>[2x]MRVLIVKTSSMGDVLHTLPALTDAQQAIPGIKFDWVVEEGFAQIPSWHAAVERVIPVAIRRWRKAWFSAPIKAERKAFREALQAKNYDAVIDAQGLVKSAALVTRLAHGVKHGMDWQTAREPLASLFYNRKHHIAKQQHAVERTRELF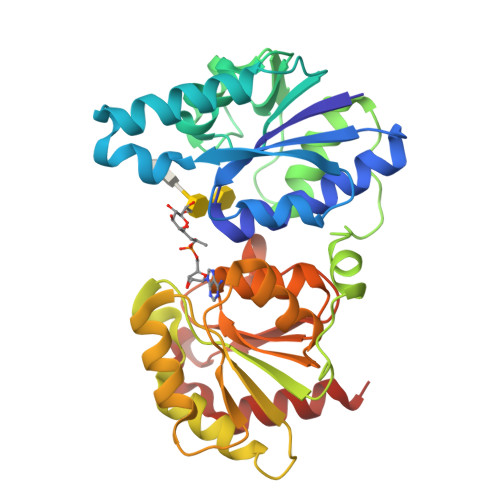AKSLGYSKPQTQGDYAIAQHFLTNLPTDAGEYAVFLHATTRDDKHWPEEHWRELIGLLADSGIRIKLPWGAPHEEERAKRLAEGFAYVEVLPKMSLEGVARVLAGAKFVVSVDTGLSHLTAALDRPNITVYGPTDPGLIGGYGKNQMVCRAPGNELSQLTANAVKQFIEENAEKAAVI>GAMGSEEKLREVSSQDPVTGLYNRSHFLDLMDAAVQQAVTARKPSTLAYIHLNGYPSLQADHGLSGIDLLLGQLAGLMREQFGEEADLARFGDSIFAALFKGKTPEQAQAALQRLLKKVENHLFELNG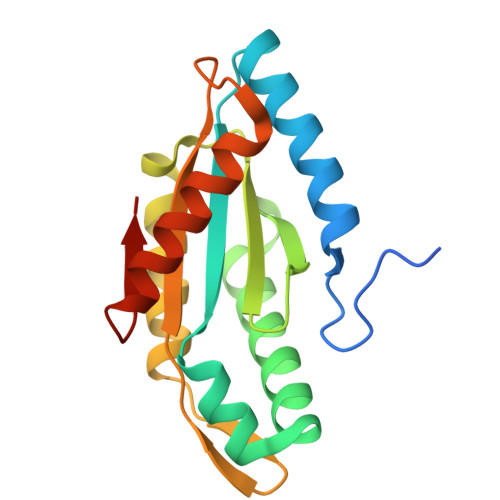RSAQATLSIGVAGLDEKTAKAQDVMNRAHRCADDAARKGGSQIKQYNPA[2x]> MADEEDPWGFDDGGEEEKAASTQAGTPAPPSKAPSVASDHKADSVVAGTPANEEAAPEEVEEIKAPPPPPEDDGYRKPVQLYRHWVRPKFLQYKYMYNYRTNYYDDVIDYIDKKQTGVAREIPRPQTWAERVLRTRNISGSDIDSYAPAKRDKQLIQTLAAS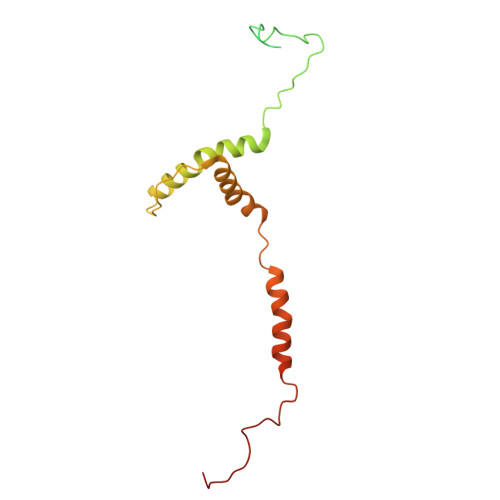IRTYNYHTKAYINQRYASVL> GPGGSMYQLEKEPIVGAETFYVDGAANRETKLGKAGYVTNRGRQKVVTLTDTTNQKTELQAIYLALQDSGLEVNIVTDSQYALGI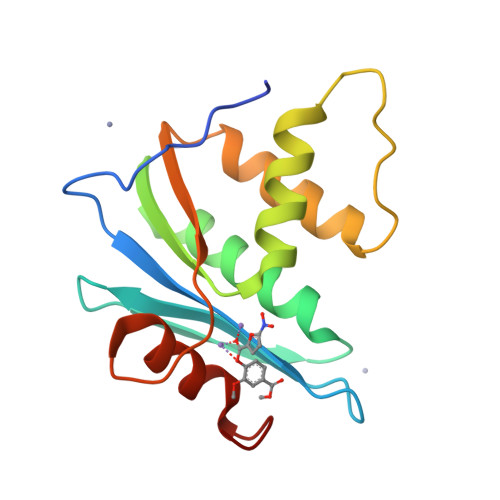ITQWIHNWKKRGWKTPVKNVDLVNQIIEQLIKKEKVYLAWVPAHKGIGGNEQVDKLVSAGIRKVLF1-(4-CHLOROPHENETHYL)-2-(2-CHLOROPHENYL)-6-OXOPIPERIDINE-3-CARBOXYLIC ACID | C20 H19 Cl2 N O3 | 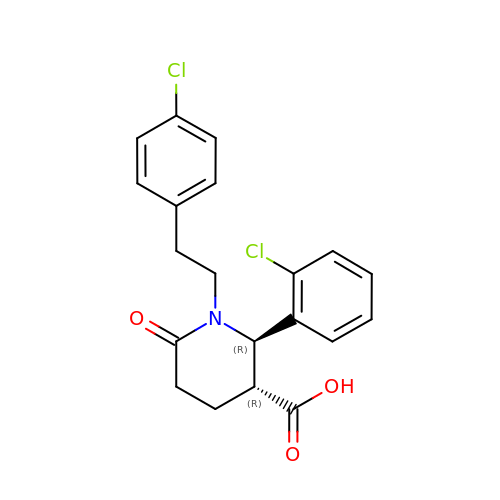HVRGSGUCGHDVGY-APWZRJJASA-N Jumonji domain-containing 7 (JMJD7) is a JmjC (3S)-lysyl-hydroxylase that catalyses the modification of Developmentally Regulated GTP Binding Proteins 1 and 2 (DRG1 and 2); JMJD7 has also been reported to have histone endopeptidase activity. Here we report biophysical and biochemical studies on JMJD7 from Drosophila melanogaster (dmJMJD7). Like hsJMJD7, dmJMJD7 forms a homodimer with each 316-amino-acid monomer possessing an N-terminal helix-loop-helix-fold domain (aa 1–42) that forms part of the dimerization interface, a core distorted double-stranded β-helix (DSBH, aa 160–294) fold comprising of eight parallel β-strands and an α-helical C-terminal domain (aa 296–310) which is also involved in dimerization. Notably, the crystallographic analyses on dmJMJD7 combined with previously reported crystal structures for hsJMJD720 reveal the unusual dimerization mode of JMJD7, which involves interactions between the N- and C-terminal regions of both dmJMJD7 monomers and is likely conserved in all animals making JMJD7.

We obtained dmJMJD7 crystals of His6-dmJMJD7.Mn complexed with its co-substrate 2OG or co-product succinate; catalytically inert Mn(II) was used instead of the cofactor Fe(II) to block catalysis under aerobic conditions, as was done for hsJMJD720. The His6-dmJMJD7.Mn structures reveal that the overall fold of dmJMJD7 is very similar to that of hsJMJD7 (root mean square deviation of 1.3 Å for Cα atoms of > 90% residues). Consistent with a higher degree of conservation of JMJD7 residues located on the DSBH core fold (~ 68%) than elsewhere, both hsJMJD7 and dmJMJD7 share almost identical active site features, an observation in accord with our biochemical observations showing their substrates are interchangeable. Like hsJMJD7, dmJMJD7 has an active site metal ion (Mn substituting for Fe) that is octahedrally coordinated by the 2OG oxalyl group, a water molecule, and the highly (but not universally) conserved metal-binding triad of residues (H175, D177, and H278). The 2OG oxoacid coordinates the metal ion with its 2-oxo carbonyl oxygen ligating trans to D177 and one of its C1 carboxylate oxygens ligating trans to H175; the other C1 carboxylate oxygen is positioned to form an H-bond with the sidechain amide of N181. The 2OG C5 carboxylate is positioned to form electrostatic/ H-bond interactions with the side-chains of four dmJMJD7 residues, Lys190 (βIV), Tyr123 (non-DSBH aa), Thr172 (βII), and Tyr183 (βIII). The conservation of 2OG C5 carboxylate binding mode of hsJMJD7 in dmJMD7 is particularly notable since this feature is uniquely characteristic of JMJD7 amongst the structurally characterised 2OG oxygenases. Notably, in the 2OG/succinate/N-oxalylglycine complexes, Trp164 is positioned to form a stacking interaction with the methylene groups of 2OG/succinate/N-oxalylglycine; the C4-methylene substitution in N-oxalyl-D-alanine or N-oxalyl-D-phenylalanine compared to N-oxalylglycine prevents this interaction.

>GSHMASMSEVERALDVLLQEAEELCIGSSVVELDRIPTALEFCREFYSKNQPVVIRKALNWPAIGKWTPKYLIEALGDRSVDVAITPNGYADGLATQNGQEYFVLPLETKMKLSEVVRRLDDPTGAVHYIQKQNSNLSVDLPELAADLRVSDLDFAQQSFNKPPDAVNFWLGDERAVTSMHKDPYENVYCVISGHKDFVLIPPHQLSCVPRGIYPTGVYKTSDSGQFYIEPLRDEEGSDQFTEWVSVDPLSPDLAKYPEYARAKPLKVRVHAGDILYLPNYWFHHVSQSHKCIAVNFWYDLDYDSRYCYYRMLEQMTSARSG[2x]>[2x]MHHHHHHSSGVDLGTENLDFEWTLKAGALEMALKRVYTLLSSWNCLEDFDQIFWGQKSALAEKVRQCWQDDELFSYQFLNGANPMLLRRSTSLPSRLVLPSGMEELRAQLEKELQNGSLFEADFILLDGIPANVIRGEKQYLAAPLVMLKMEPNGKLQPMVIQIQPPNPSSPTPTLFLPSDPPLAWLLAKSWVRNSDFQLHEIQYHLLNTHLVAEVIAVATMRCLPGLHPIFKFLIPHIRYTMEINTRARTQLISDGGIFDKAVSTGGGGHVQLLRRAAAQLTYCSLCPPDDLADRGLLGLPGALYAHDAL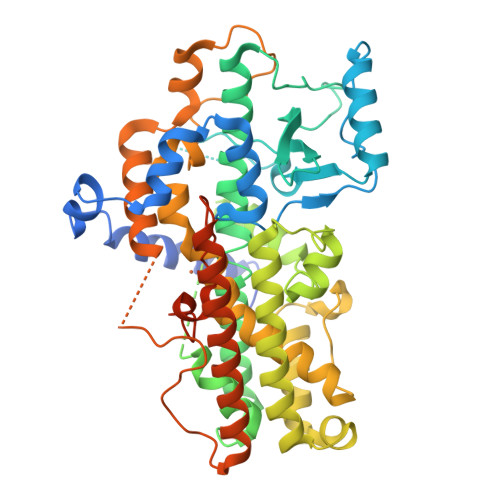RLWEIIARYVEGIVHLFYQRDDIVKGDPELQAWCREITEVGLCQAQDRGFPVSFQSQSQLCHFLTMCVFTCTAQHAAINQGQLDWYAWVPNAPCTMRMPPPTTKEDVTMATVMGSLPDVRQACLQMAISWHLSRRQPDMVPLGHHKEKYFSGPKPKAVLNQFRTDLEKLEKEITARNEQLDWPYEYLKPSCIENSVTSDSKGGYGSEFELRRQACGRTRAPPPPPLRSGC3-BENZOYL-N-[(1S,2R)-1-BENZYL-3-(CYCLOPROPYLAMINO)-2-HYDROXYPROPYL]-5-[METHYL(METHYLSULFONYL)AMINO]BENZAMIDE | 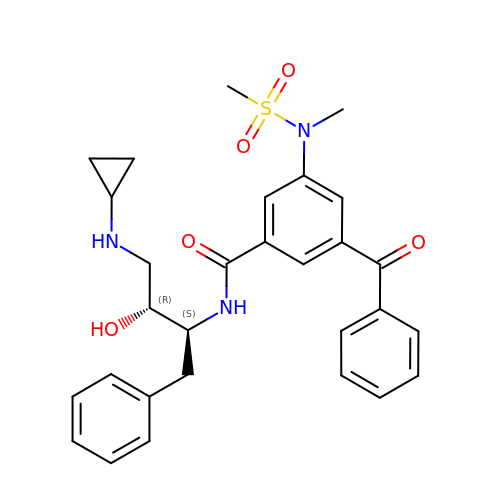C29 H33 N3 O5 S | WCVRLSCSQDAERN-RRPNLBNLSA-N> MFLINGHKQESLAVSDRATQFGDGCFTTARVIDGKVSLLSAHIQRLQDACQRLMISCDFWPQLEQEMKTLAAEQQNGVLKVVISRGSGGRGYSTLNSGPATRILSVTAYPAHYDRLRNEGITLALSPVR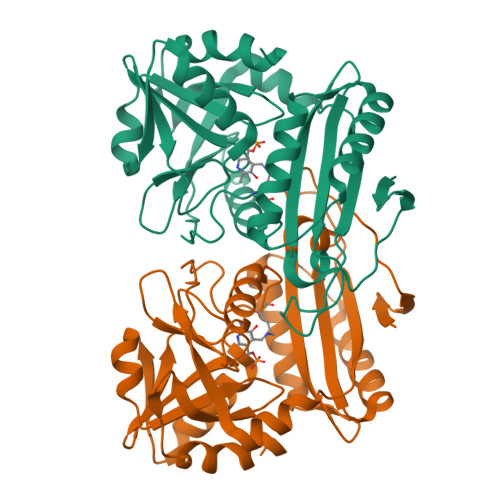LGRNPHLAGIKHLNRLEQVLIRSHLEQTNADEALVLDSEGWVTECCAANLFWRKGNVVYTPRLDQAGVNGIMRQFCIRLLAQSSYQLVEVQASLEESLQADEMVICNALMPVMPVCACGDVSFSSATLYEYLAPLCERPN>MSAQKRITLYMASASPFPHRVRLALEEAHATYEMIHISLVDKQDWYQKKVYPDRAQVPYLIYGGPELHPDEAPSPDAAKIPESLVILEFLADLFPAAHLLPSDPVLRARARLFTTAVETELLPAQKAFFLMGGPPDAMLAALDALQARLPPAGGFAAGPQWSIADAAVMPILLRLRMSVTLEVGFFAPGAAPVVRAALESPRFARLQRYIADNVARPSMAATWDEAAVKAEFVGRFEKLRSLKAAQHHHHHH[2x]

To further explore this issue, we have conducted biochemical and crystallographic studies on the interactions of six GSTOs from T. versicolor with chemical libraries. The six TvGSTOs (named TvGSTO1S to TvGSTO6S) used in this study are representatives of the twelve TvGSTOs that have a catalytic serine, while four others have a cysteine instead. In this study, we demonstrated at the biochemical and structural level that T. versicolor GSTs that belong to the Omega class interact with polyphenolic compounds found in wood, and in particular with flavonoids such as dihydrowogonin and naringenin. The ability of TvGSTOs to bind polyphenols through different sites suggests that fungal GSTs could be involved in the transport of various polyphenols.

The crystal structure of TvGSTO6S was solved at 1.45 Å resolution. As expected, it reveals the same overall fold than TvGSTO3S (rmsd 0.78 Å, 183 aligned Cα per monomer). While G-sites are made of similar polar residues, differences are observed at the H-site and at the interface between monomers. The lack of a structure with a ligand that binds in TvGSTO6S H-site precluded its fine description. However, when compared with the equivalent region of TvGSTO3S, significant differences are readily apparent in TvGSTO6S. Most of the residues that line the benzophenone binding site of TvGSTO3S are different. In addition, the extension of the C-terminal α-helix by two extra turns leads to an open and shallow H-site, contrary to the buried H-site in TvGSTO3S covered and closed by the loop corresponding to the extra turns. There are also slight differences between the dimer-interfaces of both isoforms. The larger residues of TvGSTO6S (L112 and T115 instead of T110 and A113 in TvGSTO3S) and the loss of the inter-monomer interaction between Y118 (replaced by E120 in TvGSTO6S) and E80 present in TvGSTO3S probably account for a more open dimer in TvGSTO6S. Its interface residues form a pocket centered on the two-fold axis of the dimer (rectangular section of 8 × 6 Å2), larger than the equivalent region found in TvGSTO3S (rectangular section of 7 × 4 Å2).> RS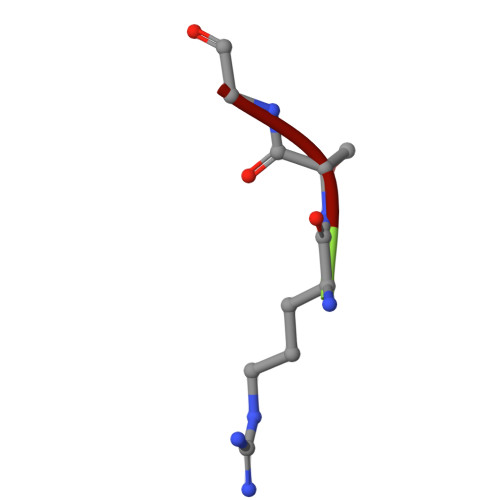G> SMQASRARLFKEYKEVQREKVADPDIQLICDDTNIFKWTALIKGPSETPYEGGVFQLAFSVPEPYPLQPPQVRFLTKIFHPNVHFKTGEICLDILKNAWSPAWTLQSVCRAIIALMAHPEPDSPLNCD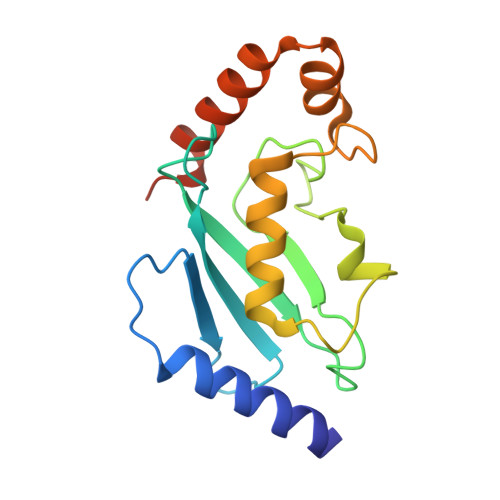SGNLLRSGDVRGFNSMAQMYTRLAAMPKKGLEVLFQ> SSDKGKLSLQDVAELIRARACQRVVVMVGAGISTPSGIPDFRSPGSGLYSNLQQYDLPYPEAIFELPFFFHNPKPFFTLAKELYPGNYKPNVTHYFLRLLHDKGLLLRLYTQNIDGLERVSGIPASKLVEAHGTFASATCTVCQRPFPGEDIRADVMADRVPRCPVCTGVVKPDIVFFGEPLPQRFLLHVVDF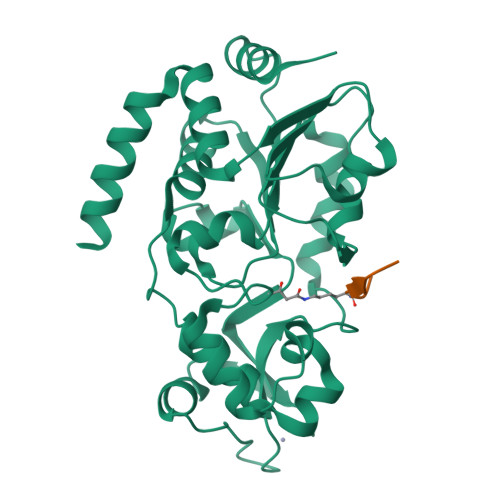PMADLLLILGTSLEVEPFASLTEAVRSSVPRLLINRDLVGPLAWHPRSRDVAQLGDVVHGVESLVELLGWTEEMRDLVQRETGKLDGPDK;> TARXSTGGKA E. coli aspartate aminotransferase (AAT) is a pyridoxal phosphate (PLP)-dependent enzyme that catalyses the reversible transamination of l-aspartate with α-ketoglutarate, yielding oxaloacetate and l-glutamate. During its catalytic cycle, AAT undergoes hinge movement to switch between an open conformation, in the ligand-free form, and a closed conformation upon association with substrates or inhibitors. Using our approach, we enrich the less populated but catalytically active closed conformation in order to increase catalytic efficiency (kcat/KM) with the non-native substrate l-phenylalanine, leading to altered substrate selectivity. Steady-state kinetics reveal kcat/KM increases of up to 100-fold towards this aromatic amino acid, resulting in a selectivity switch of up to 1900-fold, and structural analyses by room-temperature X-ray crystallography and multitemperature nuclear magnetic resonance (NMR) spectroscopy confirm that the conformational landscape is remodeled to favor the target state.

To determine if these differences in the temperature dependence of exchange could be observed in the crystal state, we also solved the maleate-free structures of WT, HEX, and VFIT at 303 K, and calculated isomorphous difference density maps by subtracting electron density at 278 K. By contrast, similar comparisons for WT and HEX showed relatively little difference density. We calculated ΔG at 278 K for HEX to be –1.72 kcal mol–1, a small difference that would be compatible with the interconversion between these two states to be part of the catalytic cycle.

>MAHHHHHHVGTFENITAAPADPILGLADLFRADERPGKINLGIGLYYDETGKIPVLTSVKKAEQYLLENETTKLYLGIDGIPEFGRCTQELLFGKGSALINDKRARTAQTPGGSGALRVAADFLAKNTSVKRVWVSNPSWPNHKSVFNSAGLEVREYAYYDAENHTLDFDALINSLNEAQAGDVVLFHGCCHNPTGIDPTLEQWQTLAQLSVEKGWLPLFDFAYQGFARGLEEDAEGLRAFAAMHKELIVASSYSKNFGLYNERVGACTLVAADSETVDRAFSQMKAAIRANYSSPPAHGASVVATILSNDALRAIWEQELTDMRQRIQRMRQLFVNTLQEKGANRDFSFIIKQNGMFSFSGLTKEQVLRLREEFGVYAVASGRVNVAGMTPDNMAPLCEAIVAVL[2x]> EQARPADDALAALGAQLFVDPALSRNATQSCATCHDPARAFTDPREGKAGLAVSVGDDGQ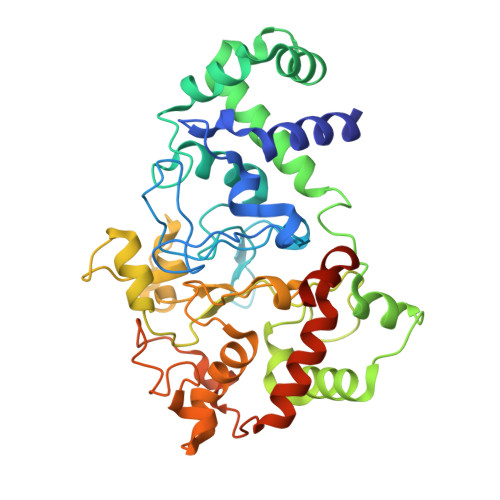SHGDRNTPTLGYAALVPAFHRDANGKYKGGQFWDGRADDLKQQAGQPMLNPVEMAMPDRAAVAARLRDDPAYRTGFEALFGKGVLDDPERAFDAAAEALAAYQATGEFSPFDSKYDRVMRGEEKFTPLEEFGYTVFITWNCRLCHMQRKQGVAERETFTNFEYHNIGLPVNETAREASGLGADHVDHGLLARPGIEDPAQSGRFKVPSLRNVAVTGPYMHNGVFTDLRTAILFHNKYTSRRPEAKINPETGAPWGEPEVARNLSLAELQSGLMLDDGRVDALVAFLETLTDRRYEPLLEESRAAQKDHHHHHH> MELPRAFGLLLHPTSLPGPYGVGVLGQEARDFLRFLKEAGGRYWQVLPLGPTGYGDSPYQSFS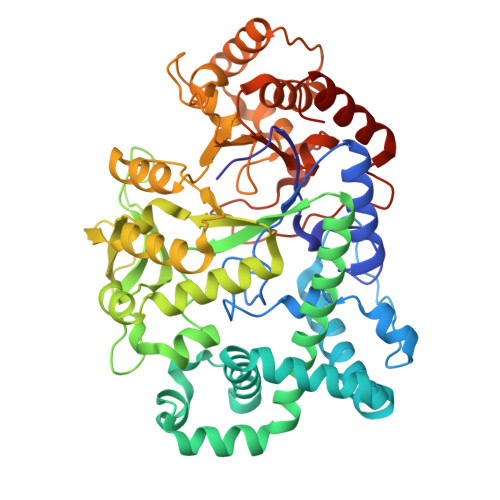AFAGNPYLIDLRPLAERGYVRLEDPGFPQGRVDYGLLYAWKWPALKEAFRGFKEKASPEEREAFAAFREREAWWLEDYALFMALKGAHGGLPWNRWPLPLRKREEKALREAKSALAEEVAFHAFTQWLFFRQWGALKAEAEALGIRIIGDMPIFVAEDSAEVWAHPEWFHLDEEGRPTVVAGVPPDYFSETGQRWGNPLYRWDVLEREGFSFWIRRLEKALELFHLVRIDHFRGFEAYWEIPASCPTAVEGRWVKAPGEKLFQKIQEVFGEVPVLAEDLGVITPEVEALRDRFGLPGMKVLQFAFDDGMENPFLPHNYPAHGRVVVYTGTHDNDTTLGWYRTATPHEKAFMARYLADWGITFREEEEVPWALMHLGMKSVARLAVYPVQDVLALGSEARMNYPGRPSGNWAWRLLPGELSPEHGARLRAMAEATERL> MHHHHHHTIVDETLNGNPEDTAHSSLSTAAARNLATTTKTVPQMQGITSRWLLRLLPWVQVSGGTYRVNRRLSHTVGDGRIDFDISGSDVAIIPEELRELPALRDFTDTEVLAALGERFTQREYAPGELIAEAGRPGDRLVLIAHGRVDRIGTGKYGDTTVLAALAGGDHLGDAPLTSDEVTWEFSYRAVTRVTVVELPRRAALEIIERSPGLREHLAGVRQGPVHPTNSSGESAVAVASGHRGEPSLPGAFADYDLAPREYELSVAQTVLRTHTRVGDLYNDPMNQVEEQLKLTVQALRERQEHEMINNREFGLLHNADLKQRIPTRSGPPTPDDLDDLLATVWKDPGFLLAHPRAIAAMAREWSARGLYPTAVDFHGHSLPSWRGVPIFPCNKIPVTKERTSSILLLRTGEEKQGVVGLHQTGIPDEYEPSLSVRFMGIDDRAVINYLVSAYYSAAVLVPDALGVLEDVEVGL

Encapsulins are a prevalent protein‐based compartmentalization strategy in prokaryotes. Family 2, the most abundant class of encapsulins, is further subdivided into Family 2A and Family 2B based on the absence or presence, respectively, of a putative cyclic nucleotide binding domain (CBD) inserted into the E‐loop of the HK97 fold encapsulin shell protein. In this work, we report the characterization of a Family 2B two‐component encapsulin shell identified in Streptomyces lydicus (Sl). Through heterologous expression and purification studies, we show the differential assembly behavior of the two shell components – Sl‐Enc1 and Sl‐Enc2 – and demonstrate their ability to co‐assemble into mixed shells with variable shell composition.

Negative stain transmission electron microscopy (TEM) analysis of purified Sl‐Enc1 and Sl‐Enc2 highlighted that Sl‐Enc1 did not assemble into regular encapsulin nanocompartments. Rather, a broad smear is observed, suggesting that Sl‐Enc1 does not assemble into homogeneous protein shells, forming irregular aggregates instead. That is to say, the Sl‐Enc1 majority sample yielded a symmetry‐averaged Sl‐Enc1 shell map while the Sl‐Enc2 majority sample resulted in a symmetry‐averaged Sl‐Enc2 shell density. As Sl‐Enc1 cannot form shells on its own, the obtained symmetry‐averaged Sl‐Enc1 map has to be treated as artifactual. However, we were able to use this map to build an atomic model of the Sl‐Enc1 protomer. First, Sl‐Enc1 exhibits a clearly defined 23‐residue N‐arm, not present in the Sl‐Enc2 protomer. The second major difference between the Sl‐Enc1 and Sl‐Enc2 protomers is that their CBDs show different relative orientations with respect to the HK97‐domain with the Sl‐Enc1 CBD being tilted by ca. 23° compared to the Sl‐Enc2 CBD. Thus, Sl‐Enc1 protomers can exist in two different states, one with clearly resolved N‐arms – as also observed in the symmetry‐averaged consensus refinement – and one with completely unresolved N‐arms. The discernable N‐arm states result in substantial differences in the size and charge of the two‐fold pores. For example, slightly unfavorable angles between Sl‐Enc1 protomer‐protomer interfaces or the presence of too many defined N‐arms – only observed for Sl‐Enc1 – could potentially propagate if too many Sl‐Enc1s are present in a given shell, resulting in an inability to form a closed compartment and a propensity toward aggregation.> VAFIGITTGLLSLATVTGNLLVLISFKVNTELKTVNNYFLLSLACADLIIGTFSMNLYTTYLLMGHWALGTLACDLWLALDYVASNASVMNLLLISFDRYFSVTRPLSYRAKRTPRRAALMIGLAWLVSFVLWAPAILFWQYLVGERTVLAGQCYIQFLSQPIITFGTAMAAFYLPVTVMCTLYWRIYRETKRAGERLAKLLEKFEALPLEDIVAALKALLATNRPEIQLAVKTIVENFP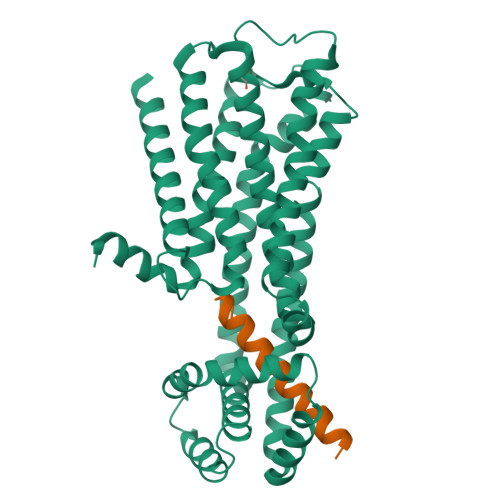EIKKEAEKLTPEQKAKLAALEAQLADLPEELRKVLLSMYLTGLLYGGSEENRKRAIEKAARTLSAILLAFILTWTPYNIMVLVSTFCKDCVPETLWELGYWLCYVNSTINPMCYALCNKAFRDTFRLLLLCR;> TPENIRFVFAAVKDTILQLNLKEYNLV>[2x]MNTDRYDSLTEVEVEGLSYLYNFADGHAYHDINEHYVDIINNLQRYWQEGKDHSIPDMEKAFKNQFAELIDSSTLHSTNHFSVCPTASNSIDIVAAWLHKENKRTALIEPAF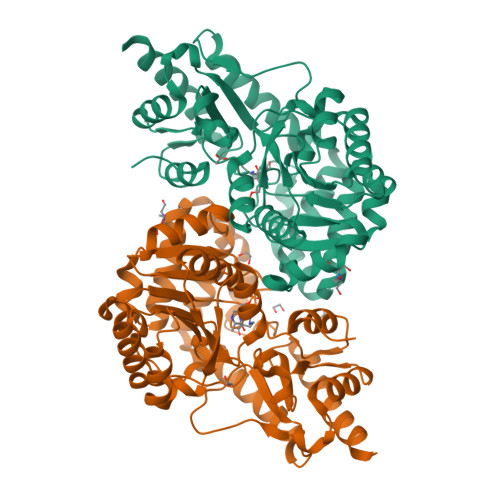DNLYLLLKRRGVDISAFDELALKNEHQLAQIVSSGDIDALFLVNPNNPTGLEMTESEFVYLVEQCKAHNITILLDRTFRIYGKTNFDDYQILEQSGIDYVVIEDTGKTWPTQDLKISLMVYSEAISSTMRLLYEEIFLCSSNFALALLKQFVAVTAKFGVDATIKNEVRRRSETINDALAGTGLKVFDNDEKCQLPLCWIDISATGYDDVSFAARLKEHDIAVLPGRFFYWNSKSQHTQFIRVSLMKPDAEFYEGIGKLKEAVTRILEKLEHHHHHH3,5-di(pyridin-4-yl)benzoic acid | C17 H12 N2 O2 | 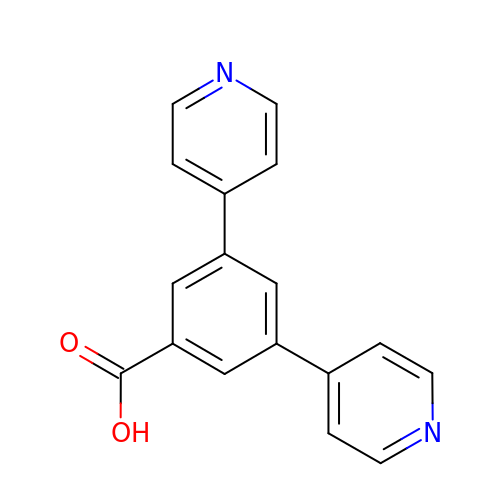NNTKTJCJOPINGZ-UHFFFAOYSA-N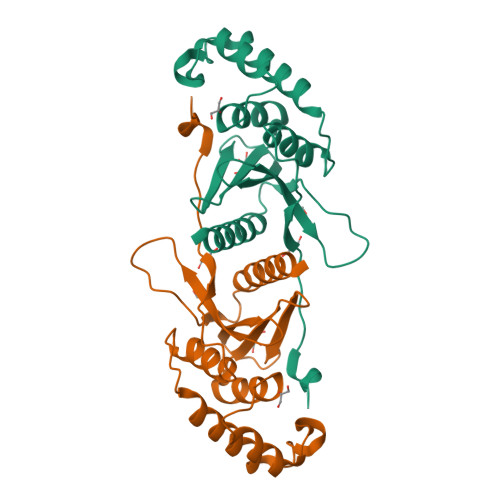> AFTKRGASSYVRETLPVLTRTVVPADNSCLFTSVYYVVEGGVLNPACAPEMRRLIAQIVASDPDFYSEAILGKTNQEYCDWIKRDDTWGGAIEISILSKFYQCEICVVDTQTVRIDRFGEDAGYTKRVLLIYDGIHYDPLQRNFPDPDTPPLTIFSSNDDIVLVQALELADEARRRRQFTDVN4-METHYLBENZYL-N-BIS[DAUNOMYCIN] | 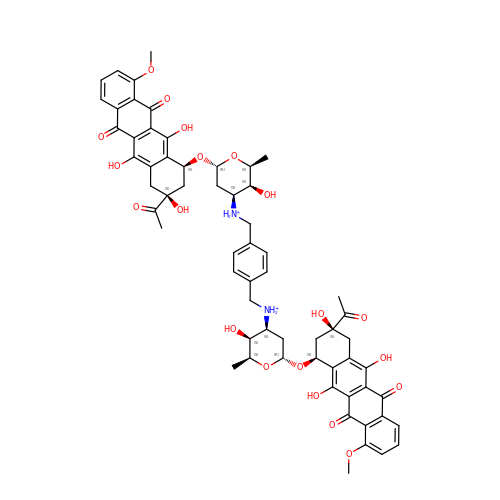C62 H66 N2 O20 | HTOLWQNKVYAHLB-MJSRGEEMSA-P>MAWDLKVKMLGGNDFLVSVTNSMTVSELKKQIAQKIGVPAFQQRLAHQTAVLQDGLTLSSLGLGPSSTVMLVVQNSSEPLSILVRNERGHSNIYEVFLTQTVDTLKKKVSQREQVHEDQFWLSFEGRPMEDKELLGEYG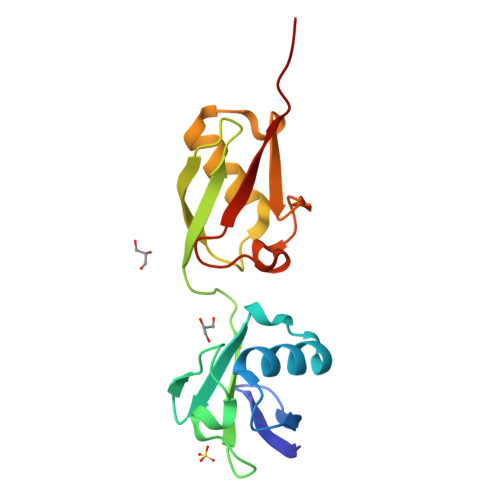LKPQCTVIKHLRLRGG[10x]> GGLVPLELSYDMTMDDLQFSMPMGVKMRNAVIMEPYMIEIDNSMEQLSFDHDE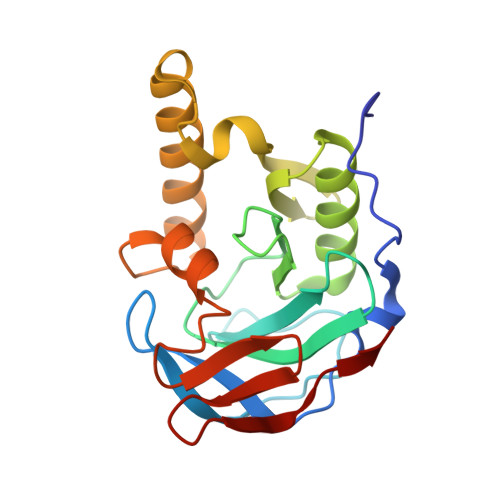SYLTMLDRHGKWRVNTMIKGFASSVQGFVSSFTTTGDIVAIGKNKADMLLAFARMKEIGGGIVLAENGNILHEIPLALCGCASSEAYEDVLEKEQKLRDLLTERGYEFCDPIYTLLFLQSTHLPYIRITPRGIFDVMKKTVLFPSIMR> ASLSFLNRSELPNLAYKRLKGKTPGIIFIPGYLSNMNGIKAVAVEEFCKSLGHAFIRFDYSGIGSSDGNLAECTVGKWRKDVLSILDDVAEGPQILVGSSLGGWLMLHAAIARPEKVIALIGIATAADGLVTQYHALPVETQKEIEMKGEWT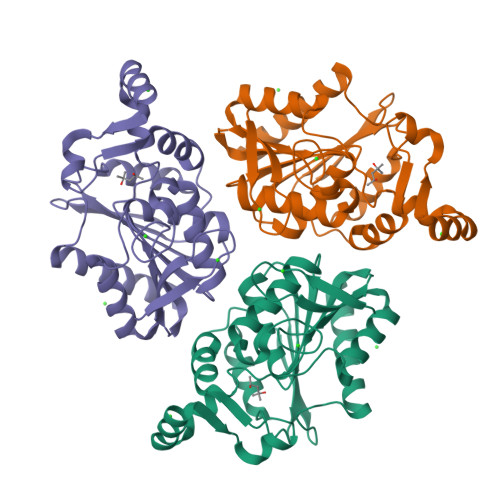LPSRYNKEGYFRIPYSFIKEAEHHCLLHSPIPVTCPVRLLHGMKDEIVPWQRSLQVADRIVSPDVDVILRKQGDHRMKEKADIHLLICTIDDLIDKLS> MHHHHHHSSGRENLYFQGSVFGVPLTVNVQRTGQPLPQSIQQAMRYLRNHCLDQVGLFRKSGVKSRIQALRQMNEGAIDCVNYEGQSAYDVADMLKQYF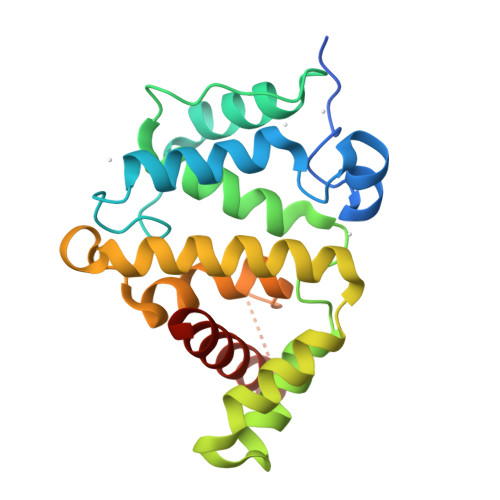RDLPEPLMTNKLSETFLQIYQYVPKDQRLQAIKAAIMLLPDENREVLQTLLYFLSDVTAAVKENQMTPTNLAVCLAPSLFHLNTLKRENSSPRVMQRKQSLGKPDQKDLNENLAATQGLAHMIAECKKL> GVDHMQTQEIISVTLQVLSLLPPYRQSISVLAGSTVEDVLKKA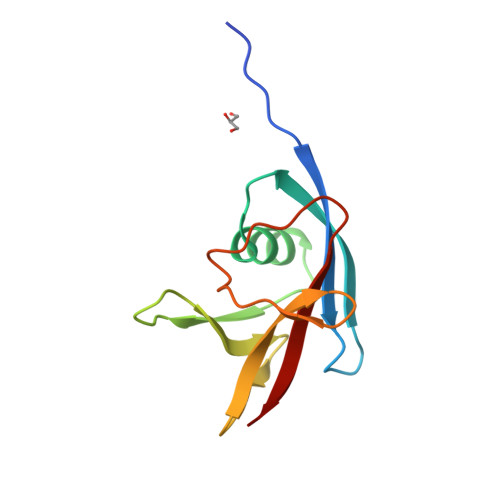HELGGFTYETQASLSGPYLTSVMGKAAGEREFWQLLRDPNTPLLQGIADYRPKDGETIELRLVSW> MTRQEELAAAR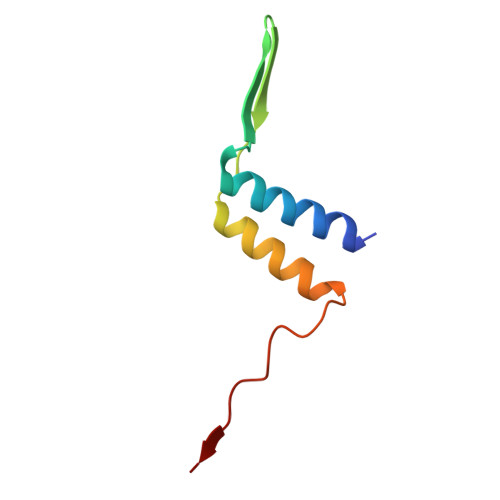AALHDLMTGKRVATVQKDGRRVEFTATSVSDLKKYIAELEVQTGMTQRRRGPAGFYV> GGSADPLRERTELLLADYLGYSAREPGTPEPAPSTPEAAVLRSAAARLRQIHRSFFSAYLGYPGNRFELVALMADSVLSDSPGPTWGRVVTLVTFAGTLLERGPLVTARWKKWGFQPRLKEQEGDVA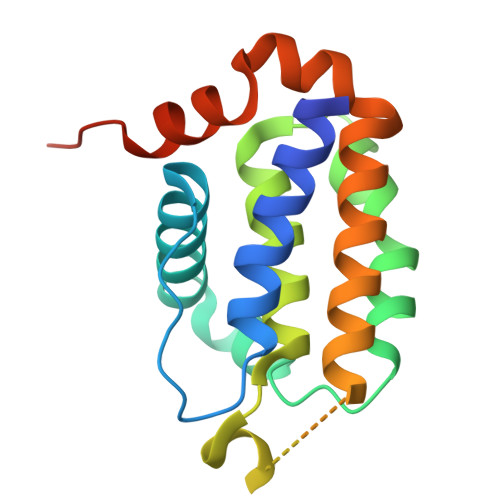RDSQRLVALLSSRLMGQHRAWLQAQGGWDGFSHFFRTPFPLAENLYFQ3-benzyladenine | C12 H12 N5 | 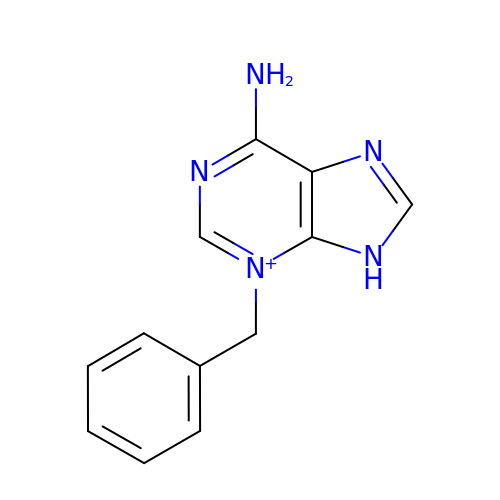SNSNPCORSVPUTC-UHFFFAOYSA-O>MSEYIRVTEDENDEPIEIPSEDDGTVLLSTVTAQFPGAC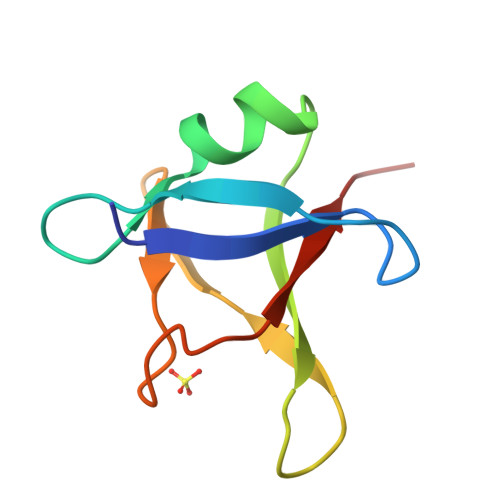GLRYRNPVSQCMRGVRLVEGILHAPDAGWGNLVYVVNYPKD[5x]>[2x]SELSFNYPNFQSVEDITFQGGASPRNETLQLTPTDSNGIPIRQRAGHAVYSQPFQLRDTSFYTTFTFVIRTTSNSPADGFAIFIAPPDFPVKRYGGYLGLFEPNTATNTSANKVVAVEFDTWVNTEWKEPRYRHIGIDVNSIVSVRVTRWQDKDVFSRSIATAHVGYDGISKILTAFVTYPDGGNYVLSHVVDLAEIFPGDVRIGFSGATGQYETQYIHSWSFSSTST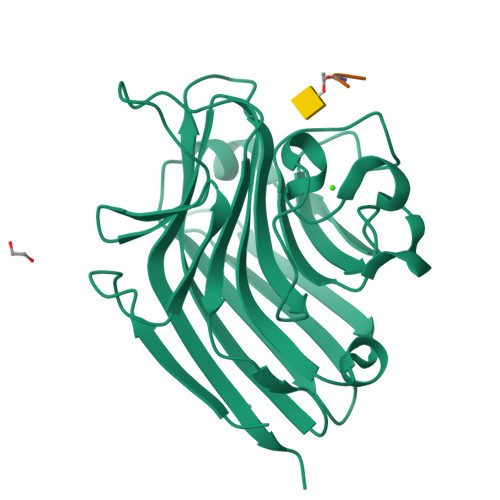NLLRDGARHHHHHH;>XSTVG[2x]>[2x]MSGADRSPNAGAAPDSAPGQAAVASAYQRFEPRAYLRNNYAPPRGDLCNPNGVGPWALRCLAQTFATGEVSGRTLIDIGSGPTVYQLLSACSHFEDITMTDFLEVNRQELGRWLQEEPGAFNWSMYSQHACLIEGKGECWQDKERQLRARVKRVLPIDVHQPQPLGAGSPAPLPADA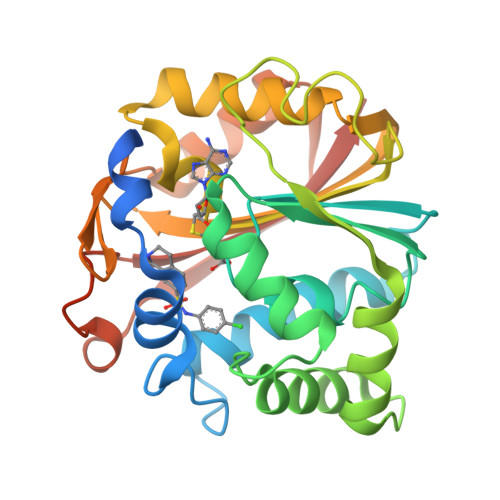LVSAFCLEAVSPDLASFQRALDHITTLLRPGGHLLLIGALEESWYLAGEARLTVVPVSEEEVREALVRSGYKVRDLRTYIMPAHLQTGVDDVKGVFFAWAQKVGLEHHHHHH>XESQL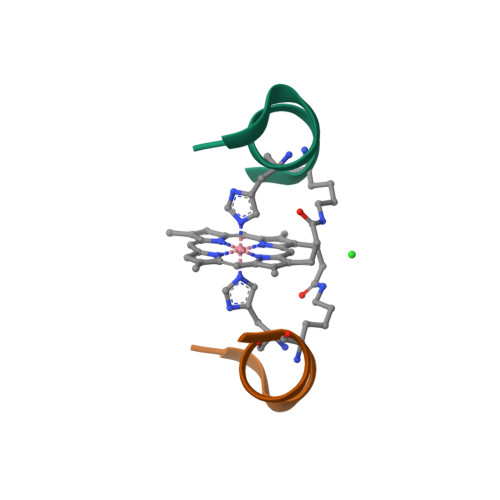HSNKRX[2x]> MKLNYFQGALYPWRFCVIVGLLLAMVGAIVWRIVDLHVIDHDFLKGQGDARSVRHIAIPAHRGLITDRNGEPLAVSTPVTTLWANPKELMTAKERWPQLAAALGQDTKLFADRIEQNAEREFIYLVRGLTPEQGEGVIALKVPGVYSIEEFRRFYPAGEVVAHAVGFTDVDDRGREGIELAFDEWLAGVPGKRQVLKDRRGRVIKDVQVTKNAKPGKTLALSIDLRLQYLAHRELRNALLENGAKAGSLVIMDVKTGEILAMTNQPTYNPNNRRNLQPAAMRNRAMIDVFEPGSTVKPFSMSAALASGRWKPSDIVDVYPGTLQIGRYTIRDVSRNSRQLDLTGILIKSSNVGISKIAFDIGAESIYSVMQQVGLGQDTGLGFPGERVGNLPNHRKWPKAETATLAYGYGLSVTAIQLAHAYAALANDGKSVPLSMTRVDRVPDGVQVISPEVASTVQGMLQQVVEAQGGVFRAQVPGYHAAGKSGTARKVSVGTKGYRENAYRSLFAGFAPATDPRIAMVVVIDEPSKAGYFGGLVSAPVFSKVMAGALRL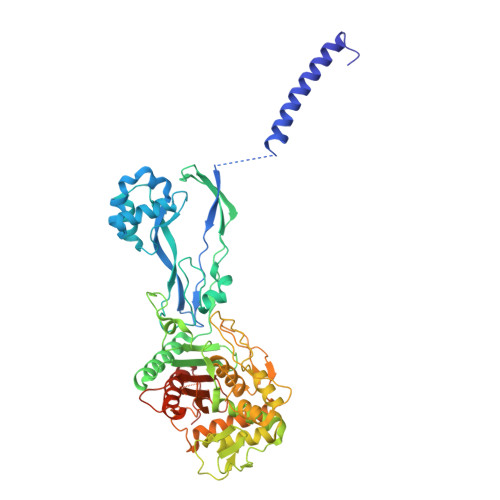MNVPPDNLPTATEQQQVNAAPAKGGRG>PYIVRLLNSSLNGCEFPLLTGRTLFVVGQSDALTASGQLPDIPADSFFIPLDHGGVNFEIQVDTDATEIILHELKEGNSESRSVQLNTPIQVG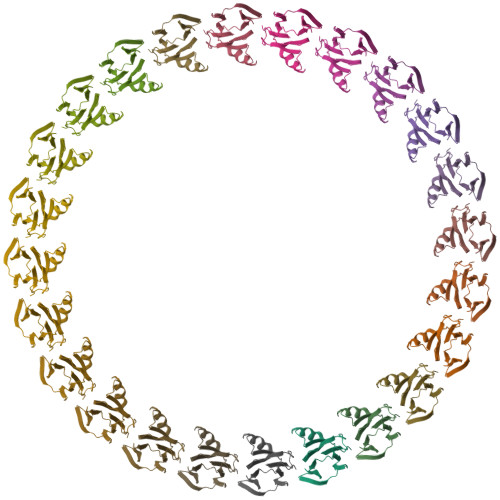ELLILIRPESEPW[24x]>[2x]AVTGPPPPLSHCGRAAPCEPLRYNVCLGSVLPYGATSTLLAGDSDSQEEAHGKLVLWSGLRNAPRCWAVIQPLLCAVYMPKCENDRVELPSRTLCQATRGPCAIVERERGWPDFLRCTPDRFPEGCTNEVQNIKFNSSGQCMVPLVRTDNPKSWYEDVEGCGIQCQNPLFTEAEHQDMHSYIAAFGAVTGLCTLFTLATFVADWRNSNRYPAVILFYVNACFFVGSIGWLAQFMDGARREIVCRADGTMRLGEPTSNETLSCVIIFVIVYYALMAGVVWFVVLTYAWHTSFKALGTTYQPLSGKTSYFHLLTWSLPFVLTVAILAVAQVDGDSVSGICFVGYKNYRYRAGFVLAPIGLVLIVGGYFLIRGVMTLFSIKSNHAKALIVYGSTTGNTEYTAETIARELADAGYEVDSRDAASVEAGGLFEGFDLVLLGCSTWGDDSIELQDDFIPLFDSLEETGAQGRKVACFGC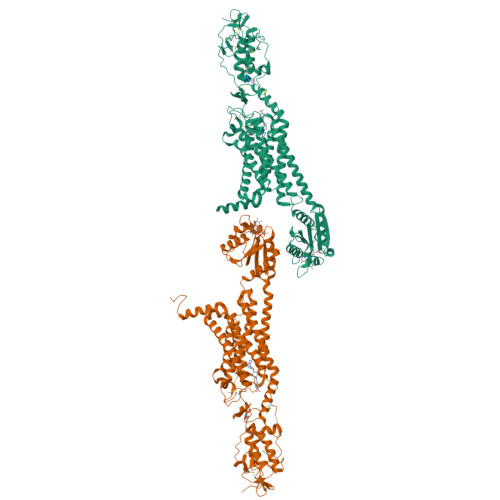GDSSWEYFCGAVDAIEEKLKNLGAEIVQDGLRIDGDPRAARDDIVGWAHDVRGAIKINETMLRLGIFGFLAFGFVLITFSCHFYDFFNQAEWERSFRDYVLCQANVTIGLPTKQPIPDCEIKNRPSLLVEKINLFAMFGTGIAMSTWVWTKATLLIWRRTWCRLTGQSDDHHHHHHHHHH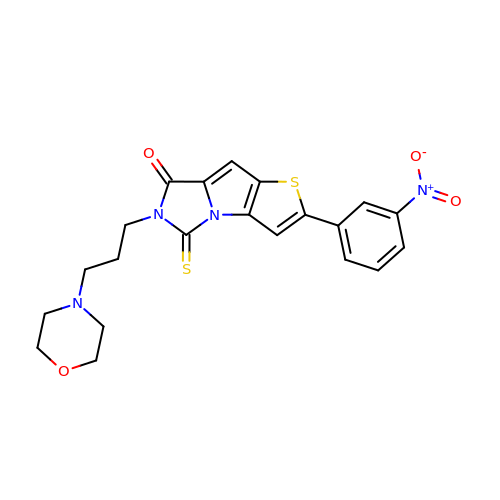5-(3-MORPHOLIN-4-YL-PROPYL)-2-(3-NITRO-PHENYL)-4-THIOXO-4,5-DIHYDRO-1-THIA-3B,5-DIAZA-CYCLOPENTA[A]PENTALEN-6-ONE | C21 H20 N4 O4 S2 | UXGUZFZBZPPZGL-UHFFFAOYSA-N> DIRAERAEQKLEPRHAMLLRCRLPGGVITTKQWQAIDKFAGENTIYGSIRLTNRQTFQFHGILKKNVKPVHQMLHSVGLDALATAWDMNRNVLCTSNPYESQLHAEAYEWAKKISEHLLPRTRAYAEIWLDQEKVATTDEEPILGQTYLPRKFKTTVVIPPQNDIDLHANDMNFVAIAENGKLVGFNLLVGGGLSIEHGNKKTYARTASEFGYLPLEHTLAVAEAVVTTQRDWGNRTDRKNAKTKYTLERV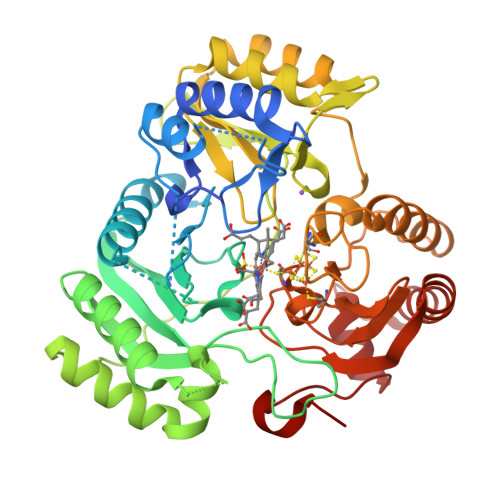GVETFKAEVERRAGIKFEPIRPYEFTGRGDRIGWVKGIDDNWHLTLFIENGRILDYPARPLKTGLLEIAKIHKGDFRITANQNLIIAGVPESEKAKIEKIAKESGLMNAVTPQRENSMACVSFPTCPLAMAEAERFLPSFIDNIDNLMAKHGVSDEHIVMRVTGCPNGCGRAMLAEVGLVGKAPGRYNLHLGGNRIGTRIPRMYKENITEPEILASLDELIGRWAKEREAGEGFGDFTVRAGIIRPVLDPARDLWD>XXXXXXXXXXXXXXXXMRWI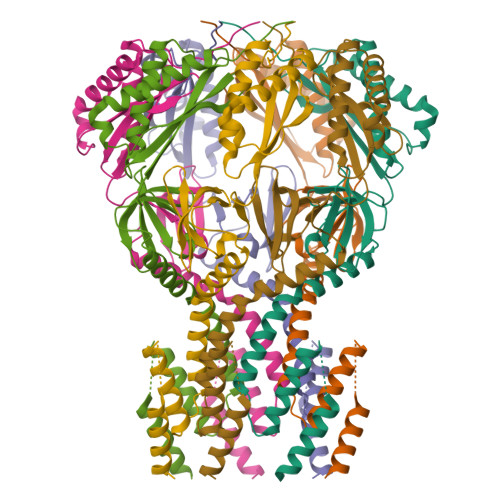LFILFCLLGAPAHAVSIPGVTTTTTTDSTTEPAPEPDIEQKKAAYGALADVLDNDTSRKELIDQLRTVAATPPAEPVPKIVPPTLVEEQTVLQKVTEVSRHYGEALSARFGQLYRNITGSPHKPFNPQTFSNALTHFSMLAVLVFGFYWLIRLCALPLYRKMGQWARQKNRERSNWLQLPAMIIGAFIIDLLLLALTLFVGQVLSDNLNAGSRTIAFQQSLFLNAFALIEFFKAVLRLIFCPNVAELRPFTIQDESARYWSRRLSWLSSLIGYGLIVAVPIISNQVNVQIGALANVIIMLCMTVWALYLIFRNKKEITQHLLNFAEHSLAFFSLFIRAFALVWHWLASAYFIVLFFFSLFDPGNSLKFMMGATVRSLAIIGIAAFVSGMFSRWLAKTITLSPHTQRNYPELQKRLNGWLSAALKTARILTVCVAVMLLLSAWGLFDFWNWLQNGAGQKTVDILIRIALILFFSAVGWTVLASLIENRLASDIHGRPLPSARTRTLLTLFRNALAVIISTITIMIVLSEIGVNIAPLLAGAGALGLAISFGSQTLVKDIITGVFIQFENGMNTGDLVTIGPLTGTVERMSIRSVGVRQDTGAYHIIPWSSITTFANFVRGIGSVVANYDVDRHEDADKANQALKDAVAELMENEEIRGLIIGEPNFAGIVGLSNTAFTLRVSFTTLPLKQWTVRFALDSQVKKHFDLAGVRAPVQTYQVLPAPGATPAEPLPPGEPTLLEHHHHHH[7x]> MESDLIDLFEGAKKAADAAALDGVTSSGPEVSQC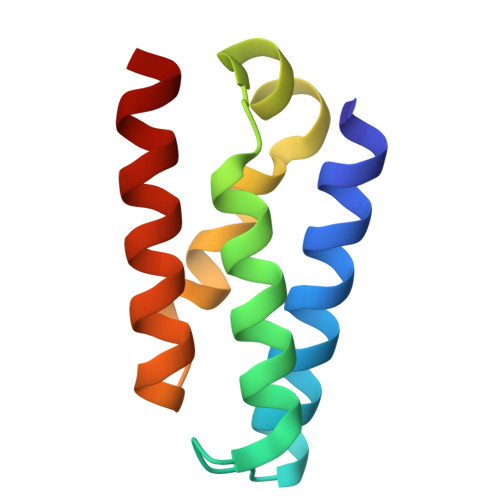IDALKQLKKFPVTYDTLVATQVGKKLRSLAKHPVEDIKSVATDLLEIWKKVVI>[4x]MGPHHHHHHLESTSLYKKAGSENLYFQGMADSKPLRTLDGDPVA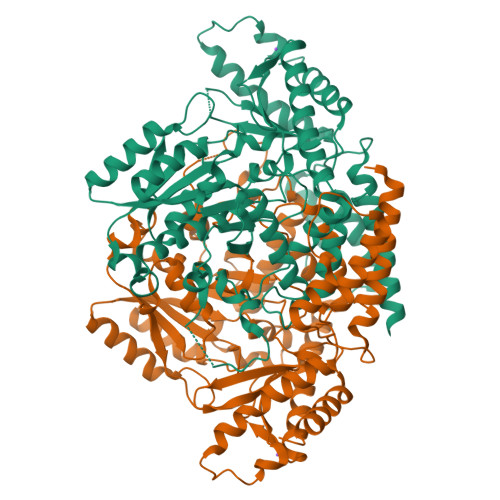VEALLQDVFGIVVDEAILKGTSASEKVCEWKEPEELKQLLDLELQSQGESREQILERCRTVIHYSVKTGHPRFFNQLFSGLDPHALAGRIITESLNTSQYTYEIAPVFVLMEEEVLKKLRALVGWNSGDGVFCPGGSISNMYAMNLARFQRYPDCKQRGLRALPPLALFTSKECHYSITKGAAFLGLGTDSVRVVKADERGRMIPEDLERQIILAEAEGSVPFLVSATSGTTVLGAFDPLDAIADVCQRHGLWFHVDAAWGGSVLLSRTHRHLLDGIQRADSVAWNPHKLLAAGLQCSALLLRDTSNLLKRCHGSQASYLFQQDKFYDVALDTGDKVVQCGRRVDCLKLWLMWKAQGGQGLERRIDQAFALTRYLVEEIKKREGFELVMEPEFVNVCFWFVPPSLRGKKESPDYSQRLSQVAPVLKERMVKKGTMMIGYQPHGTRANFFRMVVANPILAQADIDFLLGELELLGQDL>[4x]YRPISQGVSDLVGLPNQICLQKTTSTILKPRLISYTLPINTREGVCITDPLLAVDNGFFAYSHLEKIGSCTRGIAKQRIIGVGEVLDRGDKVPSMFMTNVWTPPNPSTIHHCSSTYHEDFYYTLCAVSHVGDPILNSTSWTESLSLIRLAVRPKSDSGDYNQKYIAITKVERGKYDKVMPYGPSGIKQGDTLYFPAVGFLPRTEFQYNDSNCPIIHCKYSKAENCRLSMGVNSKSHYILRSGLLKYNLSLGGDIILQFIEIADNRLTIGSPSKIYNSLGQPVFYQASYSWDTMIKLGDVDTVDPLRVQWRNNSVISRPGQSQCPRFNVCPEVCWEGTYNDAFLIDRLNWVSAGVYLNSNQTAENPVFAVFKDNEILYQVPLAEDDTNAQKTITDCFLLENVIWCISLVEIYDTGDSVIRPKLFAVKIPAQCSESG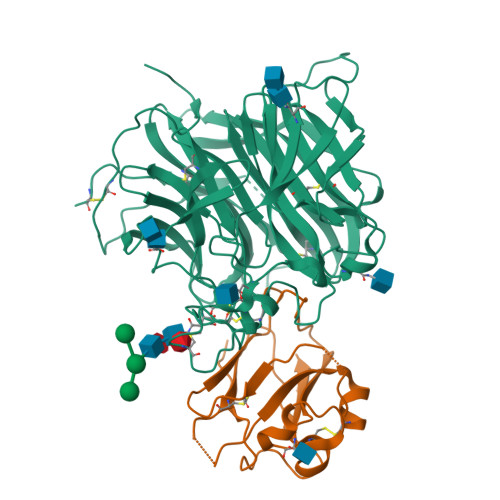RGLVPR;>SIVLEPIYWNSSNSKFLPGQGLVLYPQIGDKLDIICPKVDSKTVGQYEYYKVYMVDKDQADRCTIKKENTPLLNCAKPDQDIKFTIKFQEFSPNLWGLEFQKNKDYYIISTSNGSLEGLDNQEGGVCQTRAMKILMKVGQD[4x]2-[(3~{S})-3-azanylpiperidin-1-yl]-4-[[3-(trifluoromethyl)phenyl]amino]pyrimidine-5-carboxamide 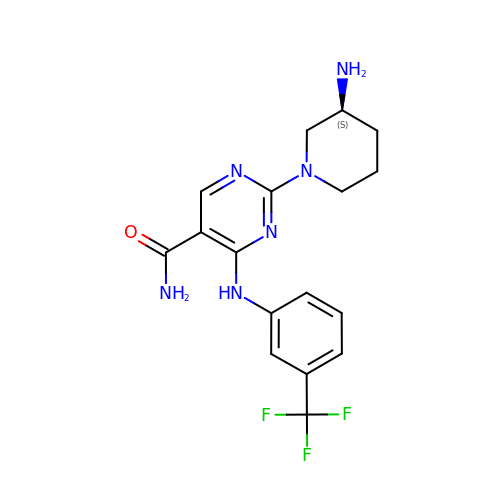| C17 H19 F3 N6 O | ASMLDRAEBPYENO-NSHDSACASA-N>[2x]GHMTIIESNYISVREEYPDIDSEVR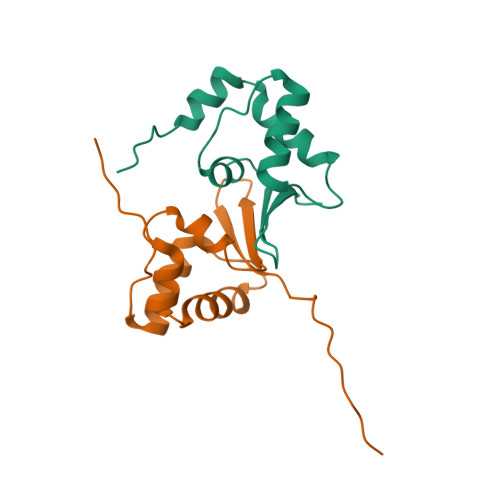AILLSHAQNGITISSIKSEYRKLTGNPFPLHDNVTDFLLTIPNVTAECSESGKRIFNLKASLKNGHLLDMVLNQKERTS> MRVLVRDLKAHVGQEVELLGFLHWRRDLGRIQFLLLRDRSGVVQVVTGGLKLPLPESALRVRGLVVENAKAPGGLEVQAKEVEVLSPALEPTPVEIPKEEWRANPDTLLEYRYVTLRGEKARAPLKVQAALVRGFRRYLDRQDFTEIFTPKVVRAGAEGGSGLFGVDYFEKRAYLAQSPQLYKQIMVGVFERVYEVA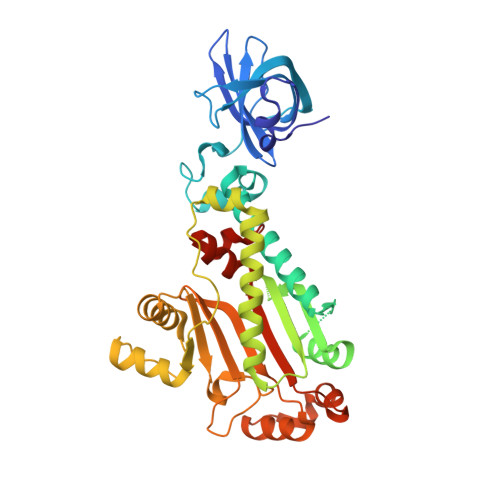PVWRMEEHHTSRHLNEYLSLDVEMGFIADEEDLMRLEEALLAEMLEEALNTAGDEIRLLGATWPSFPQDIPRLTHAEAKRILKEELGYPVGQDLSEEAERLLGEYAKERWGSDWLFVTRYPRSVRPFYTYPEEDGTTRSFDLLFRGLEITSGGQRIHRYEELLESLKAKGMDPEAFHGYLEVFKYGMPPHGGFAIGAERLTQKLLGLPNVRYARAFPRDRHRLTP> GAMGSKPDTHRADERRFLDERGSSGPLAPNGLNPATIMEKAVRERIVESYFWKEQCFGVNEADIVDRVVEHVRFVGGVTGVTQKPSPFLCLAFKLLQLAPGDDILKEYLYFGGEKFKYLRALAAFYIRLTRPDKEVYTLLE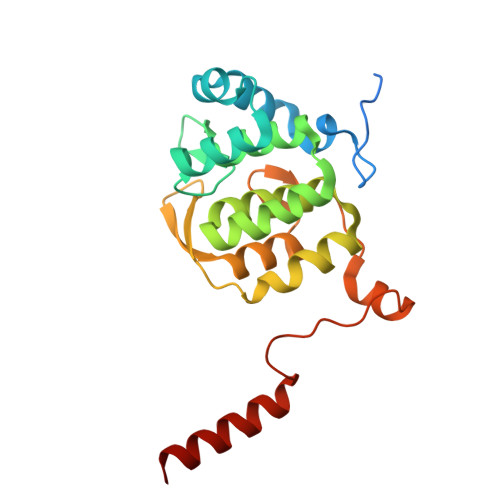PFLEDRRKLRRKGKNGTSLTYMDEFIDDLLTKDRVCSTSLWKMRRRDILEDLDLLEPRVSPLGSLEDILEEEEQAAKNEDGE> MTFAHEVVKSNVKNVKDRKGKEKQVLFNG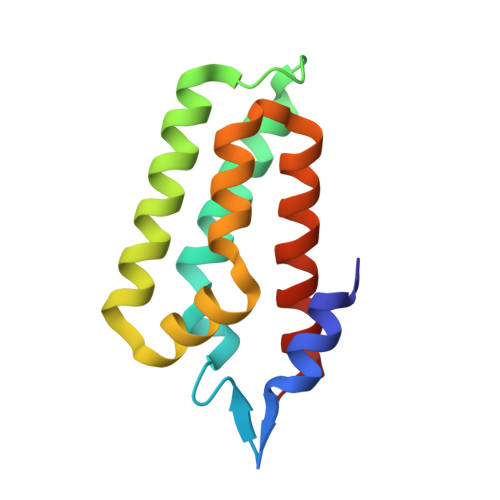LTTSKLRNLMEQVNRLYTIAFNSNEDQLNEEFIDELEYLKIKFYYEAGREKSVDEFLKKTLMFPIIDRVIKKESKKFFLDYCKYFEALVAYAKYYQKED> AAVTQSPRNKVAVTGEKVTLSCQQTNNHNNMYWYRQDTGHGLRLIHYSYGAGSTEKGDIPDGYKASRPSQEQFSLILESA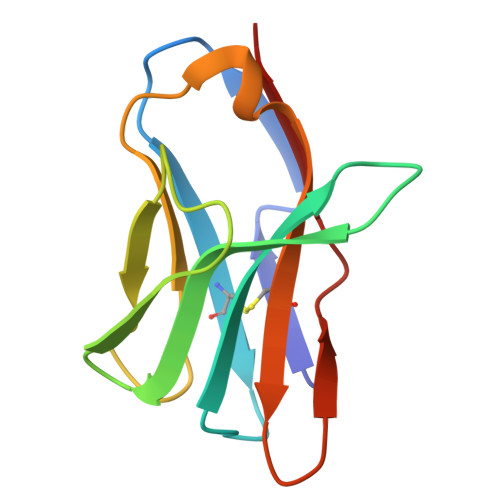TPSQTSVYFCASGGGGTLYFGAGTRLSVL> ECLVTESLKVKLQWASAFGHAHERVAFGLELWRDIIDDHPEIKAPFSRVRGDNIYSPEFGAHSQRVLSGLDITISMLDTPDMLAAQL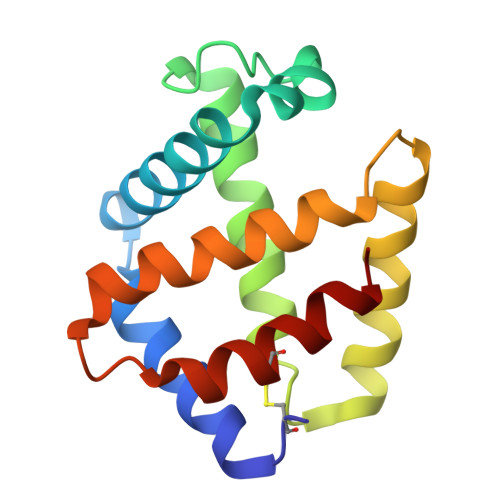AHLKVQHVERNLKPEFFDIFLKHLLHVLGDRLGTHFDFGAWHDCVDQIIDGIK> XYE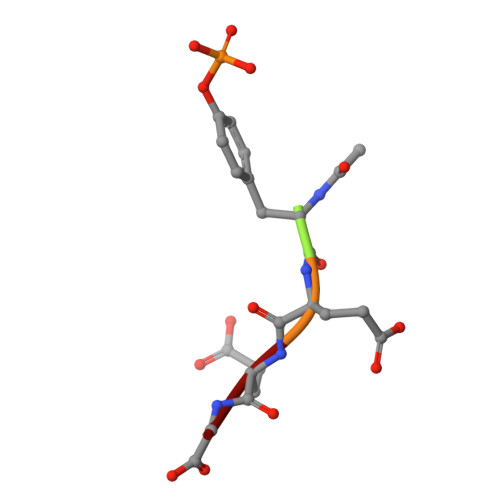EG FLASH, Flice-associated huge protein, was originally discovered as a protein involved in Fas-mediated apoptosis and later in regulation of expression of several genes, including oncogenes. Subsequent studies showed that FLASH localizes to Histone Locus Bodies in the nucleus, suggesting a role in expression of histone genes, and that it is essential for histone pre-mRNA processing. Biochemical studies revealed that the interacting N-terminal regions of Lsm11 and FLASH form a docking platform that recruits the HCC to the U7 snRNP. Our crystallographic studies of FLASH NTD demonstrate that residues 71–137 adopt a continuous and stable α-helical fold and mediate the formation of a coiled-coil dimer between two FLASH molecules.

To rule out the possibility that the observed FLASH NTD dimer is a crystallographic artifact caused by oxidized cysteine residues, we determined the structures of the FLASH NTD C54S/C83A double mutant in two different crystal forms at 2.1 and 2.6 Å resolution, respectively. In addition to Cys83, we also mutated the other Cys residue in the FLASH NTD, Cys54, in case it formed a disulfide as well even though the residue was disordered in the structure. The two structures adopt the same coiled-coil dimer as the wild-type FLASH NTD, confirming that FLASH NTD dimer formation does not require the Cys83 disulfide. The individual protomers of these two mutant dimers also show differences, similar to those observed for the wild-type dimer. Interestingly, residues 53–70 from one of the protomers in the structure at 2.6 Å resolution are stabilized by crystal packing, showing strong electron density corresponding to an α-helix. This protomer appears to form a single long α-helix from residues 53 to 137. The other protomer showed weak electron density for residues 56–62, while residues 51–55 and 63–66 are not observed. It appears that the helix for residues 53–70 does not dimerize, and it may also be structurally independent of residues 71–137, even though a single long helix (residues 53–137) is observed in one crystal form. The LDLY motif (residues 55–58) essential for binding the HCC is situated in the N-terminal helix. Whether the flexibility of this helix is a feature needed for binding the HCC will need to await further investigation.

>[2x]MSRNSLDLYEEILTEEGTAKEATYNDLQVEYGKAQLQMKELMKKFKEIQAQNFSLINENQSLKKNISALIKTARVEINRKDEEISNLHLEHHHHHH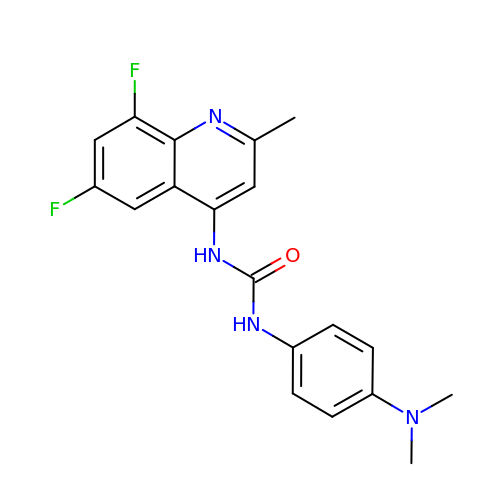1-[6,8-bis(fluoranyl)-2-methyl-quinolin-4-yl]-3-[4-(dimethylamino)phenyl]urea | C19 H18 F2 N4 O | JTARFZSNUAGHRB-UHFFFAOYSA-N methyl 6-[6-amino-2-(methylamino)-8-oxo-7,8-dihydro-1H-imidazo[4,5-g]quinazolin-4-yl]-5,6-dideoxy-beta-D-ribo-hexofuranoside 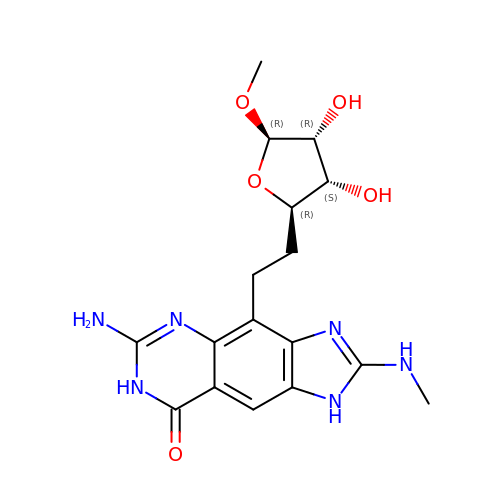| C17 H22 N6 O5 | VKQAJTKFJIETGO-QGMIFYJMSA-N>MAKKKKKKSFNVTRPTDPPVYPVTVPILGHIIQFGKSPLGFMQECKRQLKSGIFTINIVGKRVTIVGDPHEHSRFFLPRNEVLSPREVYSFMVPVFGEGVAYAAPYPRMREQLNFLAEELTIAKFQNFVPAIQHEVRKFMAANWDKDEGEINLLEDCSTMIINTACQCLFGEDLRKRLDARRFAQLLAKMESSLIPAAVFLPILLKLPLPQSARCHEARTELQKILSEIIIARKAAAVNKDSSTSDLLSGLLSAVYRDGTPMSLHEVCGMIVAAMFAGQHTSSITTTWSMLHLMHPANVKHLEALRKEIEEFPAQLNYNNVMDEMPFAERCARESIRRDPPLLMLMRKVMADVKVGSYVVPKGDIIACSPLLSHHDEEAFPEPRRWDPERDEKVEGAFIGFGAGVHKCIGQKFGLLQVKTILATAFRSYDFQLLRDEVPDPDYHTMVVGPTASQCRVKYIRRKAAAAHHHHHHHH[4x]

Trypansoma cruzi, the protozoan agent of Chagas Disease, is closely related to two other major global pathogens, Leishmania spp., responsible for leishmaniasis, and Trypansoma brucei, the causative agent of African Sleeping Sickness. Both T. cruzi and Leishmania parasites have an essential requirement for ergosterol, and are thus vulnerable to inhibitors of sterol 14α-demethylase (CYP51), which catalyzes the conversion of lanosterol to ergosterol. Here we report the crystal structures for the CYP51 target in T. cruzi (CYP51Tc) (resolutions 2.35 Å and 2.27 Å) and that of the closely related CYP51 ortholog from Trypanosoma brucei (CYP51Tb) (resolutions 2.7 Å and 2.6 Å), each bound to an anti-fungal triazole drug, either fluconazole or posaconazole. Nevertheless, CYP51Tc and CYP51Tb do share 83% sequence identity, a fact which has been crucial for successfully determining their crystal structures and makes it possible to extrapolate structural features learned from one enzyme toward the other.

The hydrophobic tunnel in CYP51Tb accommodates the antifungal drug posaconazole in either extended or bent conformations. The 2.6 Å structure of the CYP51Tb-posaconazole complex revealed four protein monomers in an asymmetric unit with posaconazole coordinating to the heme iron in a manner similar to that of fluconazole with the fluorinated edge of the 2,4-difluorophenyl ring facing away from the heme macrocycle, and the long substituent tail extending into the hydrophobic tunnel. In the CYP51Tb-posaconazole structure, four protein molecules in the asymmetric unit superimpose with the r.m.s.d. within of 0.5 Å, revealing virtually no conformational variations. However, posaconazole samples two distinct conformations due to the long tail swinging ∼7–8 Å in the hydrophobic mouth of the substrate binding tunnel. Three from the four monomers (chains A, B, and C) accommodate posaconazole in bent conformation while in the monomer D posaconazole is in extended conformation. Conformational variability of posaconazole is enabled by the interconversion of the piperazine six-membered ring between the chair and twisted boat conformations. The latter serves to accommodate the bend. Electron density is best defined in monomer B, where the terminal phenyl-2-hydroxypentan-triazolone group of posaconazole lies within 6 Å of protein residues I209-P210-A211 and V213-F214 which are invariant between CYP51Tc and CYP51Tb. In the extended conformation in monomer D, the phenyl-2-hydroxypentan-triazolone group swings toward residues I45-I46. [43], [49].The scattered Fo-Fc electron density map in the monomers A and D suggests possible interconversion of the posaconazole conformers in dynamic equilibrium, meaning that the phenyl-2-hydroxypentan-triazolone group dangles in space within the tunnel mouth.JAK2, like other JAK family members, comprises a catalytically active C-terminal tyrosine kinase domain (JH1), a regulatory pseudokinase domain (JH2), and a Src homology-2 (SH2)-like domain that, together with the N-terminal FERM (N-terminal 4.1, ezrin, radixin, moesin) domain, forms the major receptor interaction moiety. The JH2 domain has a key role in mediating both negative and positive regulation of JAK kinase activity and numerous disease mutations locate in JH2, including the prevalent hyperactivating JAK2 V617F in MPN. Previous studies have demonstrated that JAK2 JH2 binds ATP and possesses regulatory autophosphorylation activity on Ser523 and Tyr570. To gain insights on the compound binding modes to JAK2 JH2 and to analyze whether any differences could be observed between binding to WT and V617F, we determined the crystal structures of selected small molecules with JAK2 JH2 WT and V617F.

Phenylpyrazolo-pyrimidone compounds 34, 35, and 36, analogs of hit 13, engaged JAK2 JH2 domain with selectivity over JH1. The compounds that targeted JH2 domain shared a trifluoro-group as R1. Diaminotriazole analog 18, diaminotriazine compounds 4 and 24, and phenylpyrazolo-pyrimidone analogs 34 and 36 targeted JAK2 JH2 with selectivity over JH1, although the affinity of these compounds to JH2 domain was micromolar and thus lower compared to the JH1-targeting compounds 1 and 2. All compounds bind to the hinge via three hydrogen bonds (H-bonds) with the exception of 36, which makes only one hydrogen bond to the backbone amide nitrogen of Val629. Phenylpyrazolo-pyrimidone compounds identified in the present study are a novel finding for JH2-selective binders of JAK2. The affinity of phenylpyrazolo-pyrimidone compounds as well as of other JH2-selective small molecules to JAK2 JH2 was rather low, in the micromolar range.

> VFHKIRNEDLIFNESLGQGTFTKIFKGVRREVGDYGQLHETEVLLKVLDKAHRNYSESFFEAASMMSKLSHKHLVLNYGVCVCGDENILVQEFVKFGSLDTYLKKNKNCINILWKLEVAKQLAAAMHFLEENTLIHGNVCAKNILLIREEDRKTGNPPFIKLSDPGISITVLPKDILQERIPWVPPECIENPKNLNLATDKWSFGTTLWEICSGGDKPLSALDSERKLQFYEDRHQLPAPKAAELANLINNCMDYEPDHRPSFRAIIRDLNSLFTPDLVPRGSHHHHHH>MASSASGLRRGHPAGGEENMTETDAFYKREMFDPAKKYKMDHRRRGIALIFNHERFFWHLTLPERRGTCADRDNLTRRFSDLGFEVKCFNDLKAEELLLKIHEVSTVSHADADCFVCVFLSHGEGNHIYAYDAKIEIQTLTGLFKGDKCHSLVGKPKIFIIQACRGNQHDVPVIPLDVVDNQTEKLDTNITEVDAASVYTLPAGADFLMCYSVAEGYYSHRETVNGSWYIQDLCEMLGKYGSSLEFTELLTLVNRKVSQRRVDFCKDPSAIGKKQVPCFASMLTKKLHFFPKSNLEHHHHHH[4x]

Caspases belong to a highly conserved family of cysteine proteases that have essential roles in programmed cell death, inflammation, differentiation, neuronal development and axon pruning. In addition to being activated by initiator and effector caspases, Casp6 can be activated by a unique intramolecular self-cleavage mechanism due to its longer intersubunit linker. Excess neuronal active Casp6 is associated with Alzheimer disease (AD) neuropathology and age-dependent cognitive impairment. By investigating the activity of four rare natural Casp6 variants (Casp6-A34E, Casp6-E35K, Casp6-A109T, and Casp6-T182S) and employing X-ray crystallography along with molecular modelling, we have identified a putative allosteric pocket on mature active Casp6.

Following our previous work, which described rare natural Casp6-R65W and Casp6-G66R variants with significantly impaired activity, we examined four additional missense rare variants with single amino acid substitutions located remotely from Casp6 active site: Casp6-A34E, Casp6-E35K, Casp6-A109T, and Casp6-T182S. To assess the effect of mutations on Casp6 structure and function, we solved apo mature crystal structures of Casp6-E35K and Casp6-A109T but crystallisation attempts were not successful for the two other Casp6 variants. Casp6-A34E, Casp6-A109T, and Casp6-T182S did not show significant changes in kinetic parameters, KM, and kcat, for Ac-VEID-AFC hydrolysis compared with Casp6-WT, whereas Casp6-E35K displayed slightly reduced kcat and consequently showed ~2-fold reduced catalytic efficiency kcat/KM. These results suggest that E35K rare natural Casp6 substitution negatively affects Casp6 activity. In Casp6-WT the E35 from the large subunit of one protomer forms a weak salt bridge with R254 from the small subunit of the other protomer (and vice versa), stabilising the dimeric Casp6 structure. By contrast, in the Casp6-E35K, the two salt bridges are replaced by two repulsive K35-R254 pairs. In addition, E35K substitution disrupts a salt bridge between E35 from the large subunit and K284 from the small subunit of the same Casp6-WT protomer, possibly further destabilising a functional oligomeric state of Casp6. The crystal structure of apo Casp6-E35K did not reveal hints that could have elucidated a potential mechanism responsible for reduced Casp6 activity. Although E35K substitution may lead to the disruption of few intersubunit salt bridges within Casp6 dimer, we did not observe decreased in vitro stability of Casp6-E35K compared to Casp6-WT or dissociation of enzyme subunits during protein purification recently described for Caspase-9 mutant, which could provide an explanation for the enzyme inactivation. Located more than 30 Å away from either active site of the Casp6 dimer, the N-terminal loop E35 is found in the neighbourhood of K36, which together with E244 and H287 forms Zn2+-binding exosite next to the postulated allosteric pocket.Leucyl-tRNA synthetases (LeuRSs) are examples of aaRSs that rely on their editing domains to limit misaminoacylation of tRNA with near-cognate amino acids and maintain the fidelity of the genetic code. Here, we identified epetraborole (EPT) from the MMV pandemic response box as an inhibitor against the essential protein leucyl-tRNA synthetase (LeuRS) in M. abscessus. Benzoxaboroles were shown to inhibit LeuRS in fungi, gram-negative pathogens and most recently M. tuberculosis. To gain insight into the interactions between EPT and LeuRS, we solved the crystal structure of the M. abscessus editing domain (LeuRS303-498).

Comparing unliganded and liganded residues in M. abscessus editing domain structures shows a sizable shift of residues 416–422, located around the adenosine pocket, upon drug binding, including ordering of Y421 to interact with the EPT-AMP adduct phosphate, and a decrease of B factors in the neighbouring residues. This increase in order could explain the relatively lower entropic contribution to binding observed in ITC, although an unliganded M. tuberculosis structure is not available for comparison.

> SQGASVLFGAPGAGDIEVFTTRPDTLFGATYMVLAPEHPLVDQLAADVWPQDTDPRWTGGQDSPRAAIEQYRRSIAAKSDLERQENKEKTGVFTGAYATNPVSGKPVPVFIADYVLLGYGTGAIMAVPGHDQRDWDFANTFGLPVQEVISGGDVTKAAYTGDGVLVNSDYLDGLDIEAAKVEVTRRLVKDGRGESR> GGGUUAUGUGUGCCCGGCAUGGGUGCAGUCUAUAGGGUGAGAGUCCCGAACUGUGAAGGCAGAAGUAACAGUUAGCCUAACGCAAGGGUGUCCGUGGCGACAUGGAAUCUGAAGGAAGCGGACGGCAAACCUUCGGUCUGAGGAACACGAACUUCAU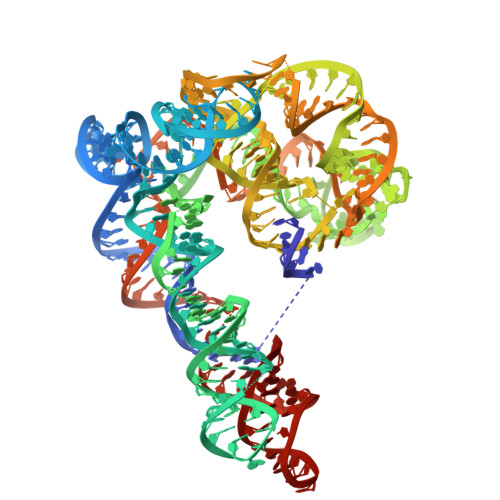AUGAGGCUAGGUAUCAAUGGAUGAGUUUGCAUAACAAAACAAAGUCCUUUCUGCCAAAGUUGGUACAGAGUAAAUGAAGCAGAUUGAUGAAGGGAAAGACUGCAUUCUUACCCGGGGAGGUCUGGAAACAGAAGUCAGC>[2x]MVRRTKEEAQETRAQIIEAAERAFYKRGVARTTLADIAE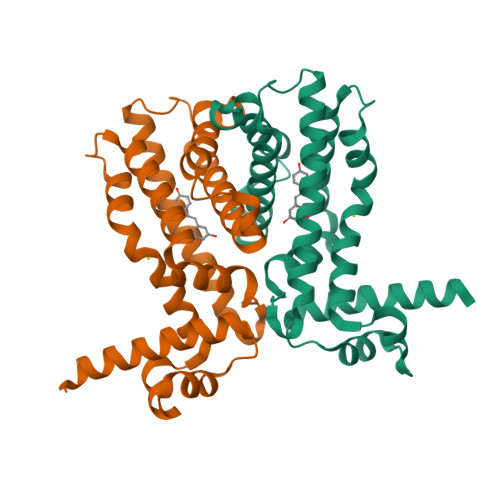LAGVTRGAIYWHFNNKAELVQALLDSLHETHDHLARASESEDEVDPLGCMRKLLLQVFNELVLDARTRRINEILHHKCEFTDDMCEIRQQRQSAVLDCHKGITLALANAVRRGQLPGELDAERAAVAMFAYVDGLIRRWLLLPDSVDLLGDVEKWVDTGLDMLRLSPALRK> TPASRYITDMTIEELSRDWFMLMPKQKVEGPLCIRIDQAIMDKNIMLKANFSVIFDRLETLILLRAFTEEGAIVGEISPLPSFPGHTIEDVKNAIGVLIGG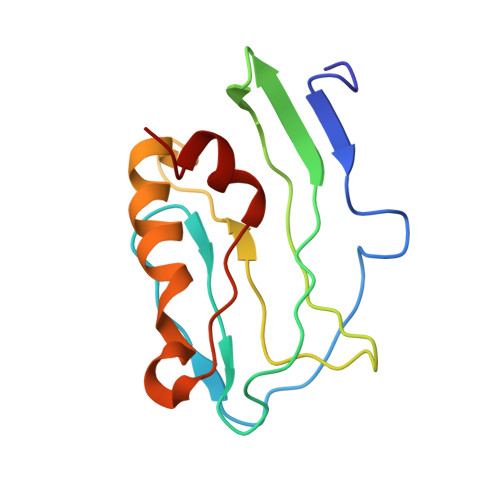LEWNDNTVRVSKTLQRFAWGS> MTSGSALF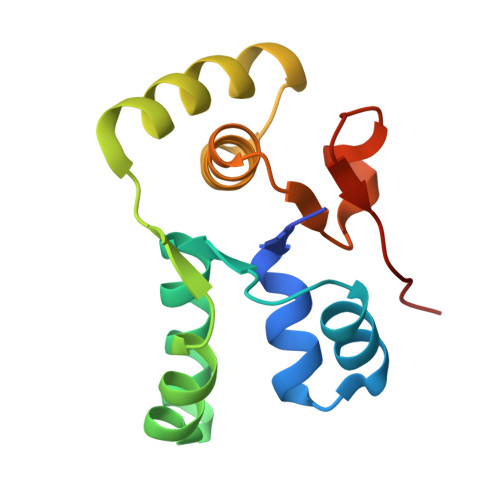DTNILIDLFSGRREAKQALEAWPPQNAISLITWMEVMVGAKKYHQEQRTRMALSTFNIINISQDIAERSVALRQEYKLKLPDAIILATAQLHRLELITRNTKDFAGIPGVVTPYEIHPE> GPLGSVWQLISKVLARHFSAADASRVLEQLQRDYERSLSRLTLDDIERLASRFLHPEV;> GPLGSAKRRKTMQGEGPQ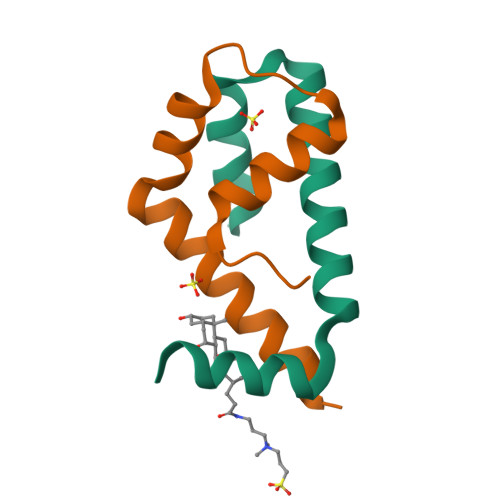LLLSEAVSRAAKAAGARPLTSPESLSRDLEAPEVQESYRQQLRSDIQKRLQEDPNYSPQRFPN> XYK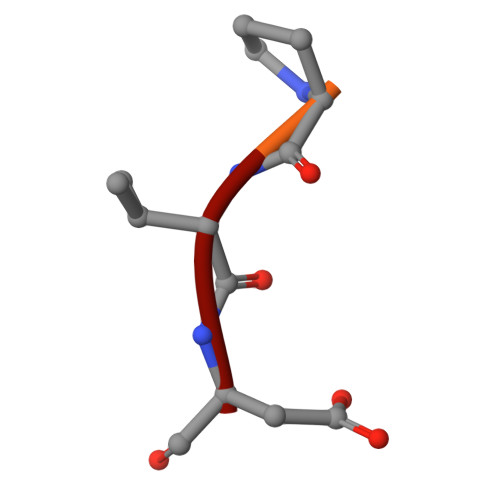PVD> MKSVITT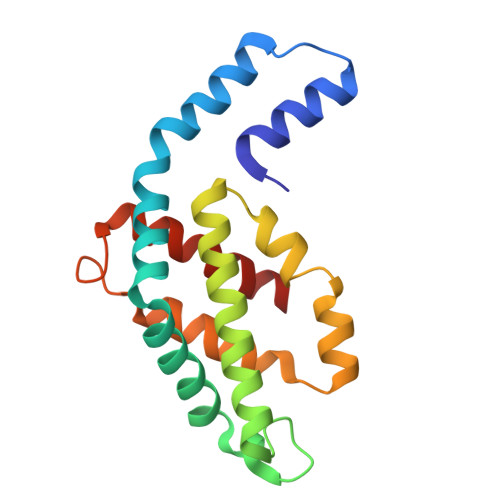VVSAADAAGRFPSNSDLESIQGNIQRSAARLEAAEKLAGNHEAVVKEAGDACFAKYAYLKNPGEAGENQEKINKCYRDVDHYMRLVNYCLVVGGTGPLDEWGIAGAREVYRTLNLPTSAYVASIAYTRDRLCVPRDMSAQAGVEFSAYLDYLINALS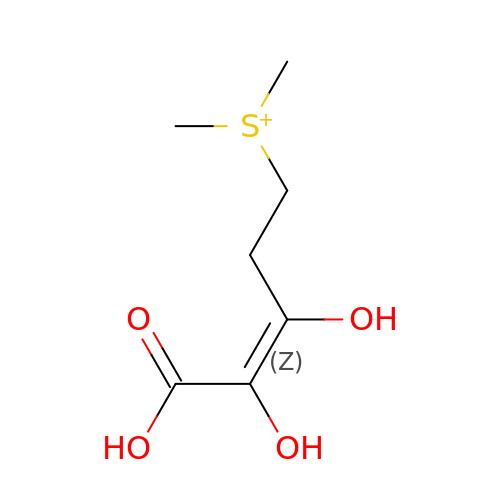dimethyl-[(Z)-3,4,5-tris(oxidanyl)-5-oxidanylidene-pent-3-enyl]sulfanium | C7 H13 O4 S | OURROQZHBYSLDP-WAYWQWQTSA-O>[2x]MAISLATKAATDALKVNRAPVGVEPQEVHKWLQSFNWDFKENRTKYPTKYHMANETKEQFKVIAKEYARMEAAKDERQFGTLLDGLTRLGAGNKVHPRWGETMKVISNFLEVGEYNAIAASAMLWDSATAAEQKNGYLAQVLDEIRHTHQCAFINHYYSKHYHDPAGHNDARRTRAIGPLWKGMKRVFADGFISGDAVECSVNLQLVGEACFTNPLIVAVTEWASANGDEITPTVFLSVETDELRHMANGYQTVVSIANDPASAKFLNTDLNNAFWTQQKYFTPVLGYLFEYGSKFKVEPWVKTWNRWVYEDWGGIWIGRLGKYGVESPASLRDAKRDAYWAHHDLALAAYAMWPLGFARLALPDEEDQAWFEANYPGWADHYGKIFNEWKKLGYEDPKSGFIPYQWLLANGHDVYIDRVSQVPFIPSLAKGTGSLRVHEFNGKKHSLTDDWGERQWLIEPERYECHNVFEQYEGRELSEVIAEGHGVRSDGKTLIAQPHTRGDNLWTLEDIKRAGCVFPDPLAKF;>[2x]MSQPQSSQVTKRGLTDPERAAIIAAAVPDHALDTQRKYHYFIQPRWKRLSEYEQLSCYAQPNPDWIAGGLDWGDWTQKFHGGRPSWGNESTELRTTDWYRHRDPARRWHHPYVKDKSEEARYTQRFLAAYSSEGSIRTIDPYWRDEILNKYFGALLYSEYGLFNAHSSVGRDCLSDTIRQTAVFAALDKVDNAQMIQMERLFIAKLVPGFDASTDVPKKIWTTDPIYSGARATVQEIWQGVQDWNEILWAGHAVYDATFGQFARREFFQRLATVYGDTLTPFFTAQSQTYFQTTRGAIDDLFVYCLANDSEFGAHNRTFLNAWTEHYLASSVAALKDFVGLYA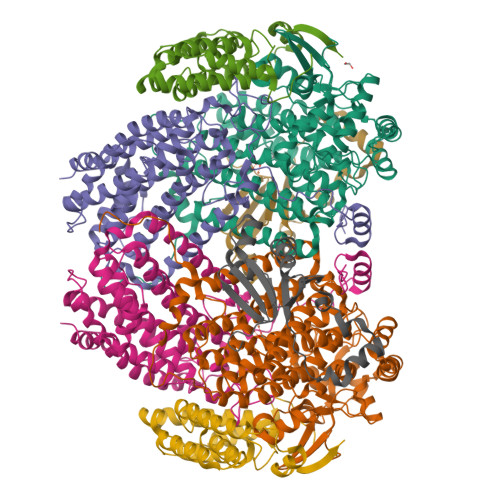KVEKVAGATDRAGVSEALQRVFGDWKIDYADKIGFRVDVDQKVDAVLAGYKN;>MAKREPIHDNSIRTEWEAKIAKLTSVDQATKFIQDFRLAYTSPFRKSYDIDVDYQYIERKIEEKLSVLKTEKLPVADLITKATTGEDAAAVEATWIAKIKAAKSKYEAERIHIEFRQLYKPPVLPVNVFLRTDAALGTVLMEIRNTDYYGTPLEGLRKERGVKVLHLQA[2x];>MSSAHNAYNAGIMQKTGKAFADEFFAEENQVVHESNAVVLVLMKSDEIDAIIEDIVLKGGKAKNPSIVVEDKAGFWWIKADGAIEIDAAEAGELLGKPFSVYDLLINVSSTVGRAYTLGTKFTITSELMGLDRALTDI[2x]>[8x]SMTVPSN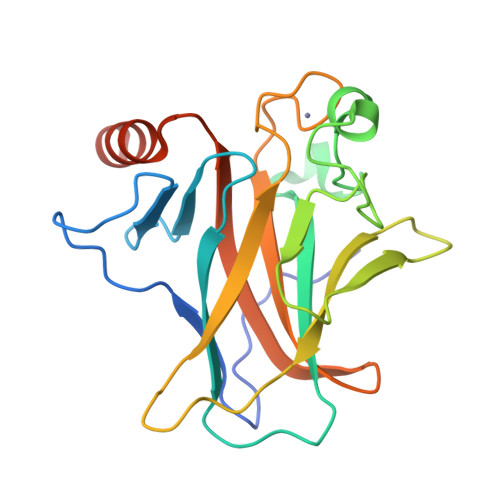TPYSGEYGFEISFQHQSKETKSTTWTFSESLKKLFVRMATTCPVRFKTVHQPPAGSVIRAMPIYVKPEHVQEVVKRCPNHATTKEHNEDHPAPTHLVRCEHKLASYVEDPYTGRQSVIIPQEHPQAGAEWVTNLYQFMCFSSCVGGLNRRPIQVIFTLEHEGVVLGRQAVEVRICACPGRDRRAEETAADPNKQQKR5-(1-{[2-(difluoromethoxy)phenyl]methyl}-2-{[3-(2-oxopyrrolidin-1-yl)phenoxy]methyl}-1H-benzimidazol-6-yl)pyridin-2(1H)-one 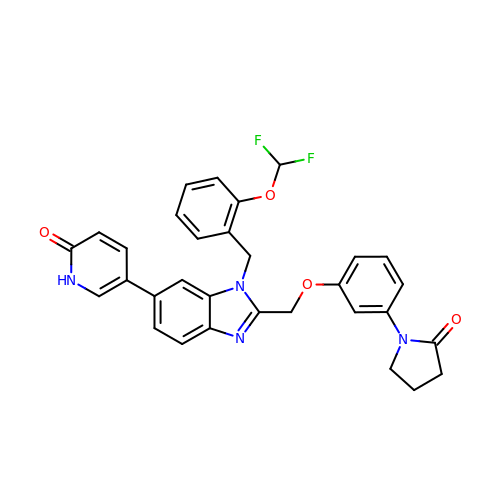| C31 H26 F2 N4 O4 | DNTKSNFCNRDJAC-UHFFFAOYSA-N> SWKVKEIVIMSVISIVFAVVYLLFTHFGNVLAGMFGPIAYEPIYGIWFIVSVIAAYMIRKPGAALVSEIIAALVECLLGNPSGPMVI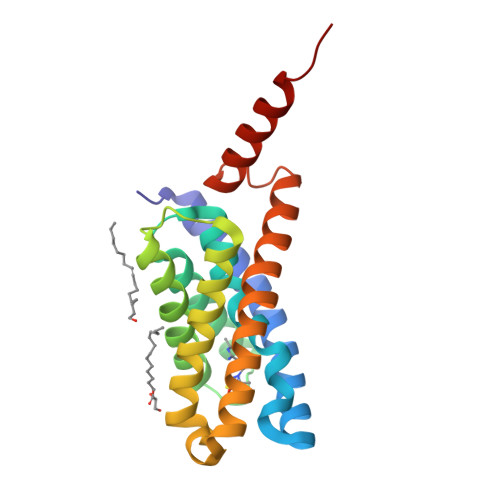VIGIVQGLGAEAVFLATRWKAYSLPVLMLAGMGSSVASFIYDLFVSGYAAYSPGYLLIMLVIRLISGALLAGLLGKAVSDSLAYTGVLNGMALGKELKKKRKRASEHASL asiatic acid | C30 H48 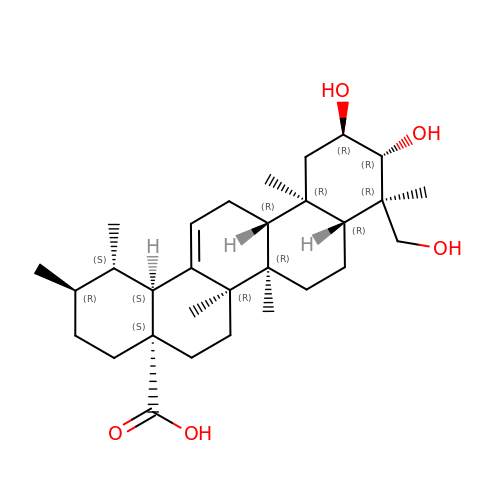O5 | JXSVIVRDWWRQRT-UYDOISQJSA-N>MEYRYDDNATNVKAMKYLIEHYFDNFKVDSIEIIGSGYDSVAYLVNNEYIFKTKFSTNKKKGFAKEKAIYNFLNTNLETNVKIPNIEYSYISDELSILGYKEIKGTFLTPEIYSTMSEEEQNLLKRDIASFLRQMHGLDYTDISECTIDNKQNVLEEYILLRET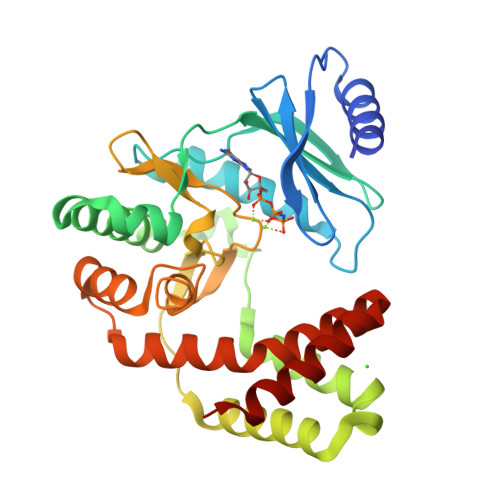IYNDLTDIEKDYIESFMERLNATTVFEGKKCLCHNDFSCNHLLLDGNNRLTGIIDFGDSGIIDEYCDFIYLLEDSEEEIGTNFGEDILRMYGNIDIEKAKEYQDIVEEYYPIETIVYGIKNIKQEFIENGRKEIYKRTYKD[4x]>PEVGELIEKVRKAHQETFPALCQLGKYTTNNSSEQRVSLDIDLWDKFSELSTKCIIKTVEFAKQLPGFTTLTIADQITLLKAACLDILILRICTRYTPEQDTMTFSDGLTLNRTQMHNAGFGPLTDLVFAFANQLLPLEMDDAETGLLS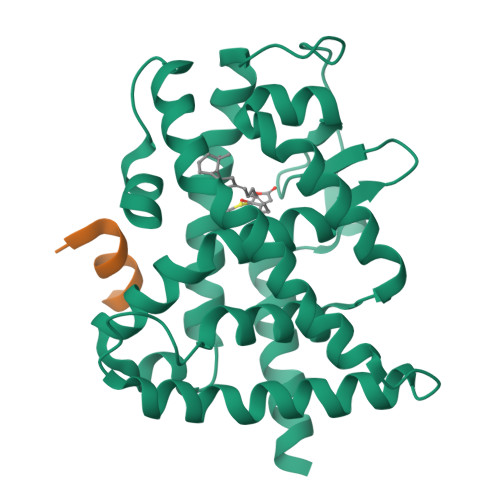AICLICGDRQDLEQPDRVDMLQEPLLEALKVYVRKRRPSRPHMFPKMLMKITDLRSISAKGAERVITLKMEIPGSMPPLIQEMLE[2x];>KSLLQQLLTE[2x]>[2x]GSANDSPAKSLVDIDLSSLRDPAGIFELVEVVGNGTYGQVYKGRHVKTGQLAAIKVMDVTEDEEEEIKLEINMLKKYSHHRNIATYYGAFIKKSPPGHDDQLWLVMEFCGAGSITDLVKNTKGNTLKEDWIAYISREILRGLAH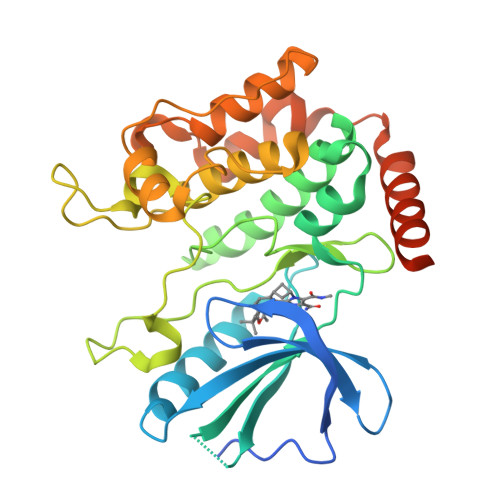LHIHHVIHRDIKGQNVLLTENAEVKLVDFGVSAQLDRTVGRRNTFIGTPYWMAPEVIACDENPDATYDYRSDLWSCGITAIEMAEGAPPLCDMHPMRALFLIPRNPPPRLKSKKWSKKFFSFIEGCLVKNYMQRPSTEQLLKHPFIRDQPNERQVRIQLKDHIDRTRKKRGEKDETEYEYSGSEEGNS>XEVEALEKKVEALEYKVQKLEKKVEALEHGWD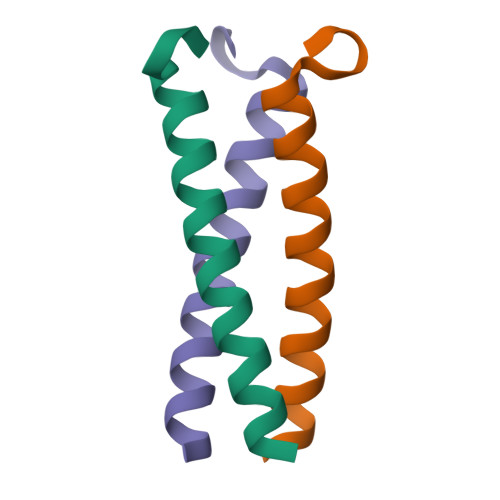GR[2x]>[4x]GPHMAAAAMAAAAGGGAGAARSLSRFRGCLAGALLGDCVGSFYEAHDTVDLTSVLRHVQSLEPDPGTPGSERTEALYYTDDTAMARALVQSLLA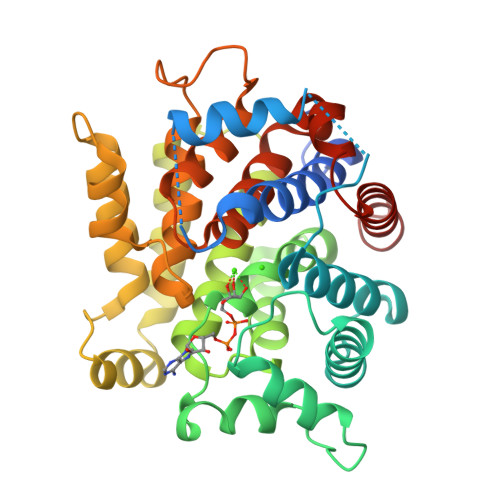KEAFDEVDMAHRFAQEYKKDPDRGYGAGVVTVFKKLLNPKCRDVFEPARAQFNGKGSYGNGGAMRVAGISLAYSSVQDVQKFARLSAQLTHASSLGYNGAILQALAVHLALQGESSSEHFLKQLLGHMEDLEGDAQSVLDARELGMEERPYSSRLKKIGELLDQASVTREEVVSELGNGIAAFESVPTAIYCFLRCMEPDPEIPSAFNSLQRTLIYSISLGGDTDTIATMAGAIAGAYYGMDQVPESWQQSCEGYEETDILAQSLHRVFQKS> MSDSHHKPVWDRTHHAKMATGIGDPQCFKGMAGKSKFNVGDRVRIKDLPDLFYTRTMTYTRGATGTIVRLVYESPAAEDEAFG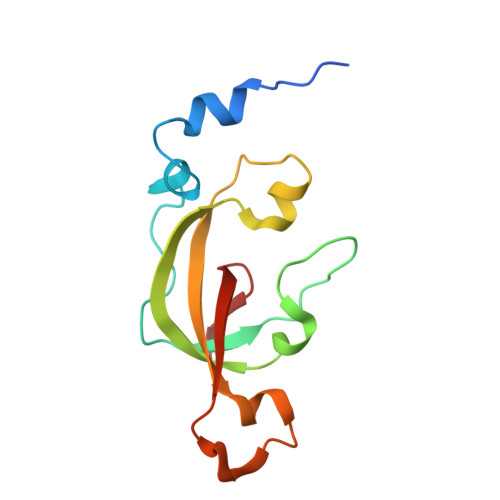NEENVEWFYSIVFAQKDLWPEYSDTFANDTLETEIPERYLEKA> GTMGVNAVHWFRKGLRLHDNPALKECIQGADTIRCVYILDPWFAGSSNVGINRWRFLLQCLEDLDANLRKLNSRLFVIRGQPADVFPRLFKEWNITKLSIEYDSEPFGKERDAAIKKLATEAGVEVIVRISHTLYDLDKIIELNGGQPPLTYKRFQTLVSKMEPLEMPADTITSDVIGKCMTPLSDDHDEKYGVPSLEELGFDTDGLSSAVWPGGETEALTRLERHLERKAWVANFERPRMNANSLLASPTGLSPYLRFGCLSCRLFYFKLTDLYKKVKKNSSPPLSLYGQLLWREFFYTAATNNPRFDKMEGNPICVQIPWDKNPEALAKWAEGRTGFPWIDAIMTQLRQEGWIHHLARHAVACFLTRGDLWISWEEGMKVFEELLLDADWSINAGSWMWLSCSSFFQQFFHCYCPVGFGRRTDPNGDYIRRYLPVLRGFPAKYIYDPWNAPEGIQKVAKCLIGVNYPKPMVNHAEASRLNIERMKQIYQQLSRYRG

1 This clock is composed of a transcriptional regulatory network of clock genes, Period ( Per1 and Per2), Cryptochrome ( Cry1 and Cry2), Clock and Bmal1. In the core feedback loop of the mammalian circadian clock, transcription factors CLOCK and BMAL1 activate transcription of Per and Cry genes by forming a heterodimer. The translated PER and CRY proteins then repress the transcriptional activity of CLOCK-BMAL1 to close the loop, followed by the degradation of PER and CRY through the ubiquitin-proteasome pathway reactivating CLOCK-BMAL1. 31 CRY is a repressor of CLOCK-BMAL1, and CRY stabilization reduces the expression of CLOCK-BMAL1-target genes such as Per2.

In this study, we revealed the effects of a new circadian clock modulator TH401, which contains a methylbenzimidazole moiety, on CRY isoforms by taking a target-based approach. TH401 directly interacted with CRY1 and CRY2, albeit with a slight preference to CRY2, and the X-ray crystal structure of a CRY1-TH401 complex revealed the binding mode of TH401. The overall protein fold was highly similar to previously published CRY1 structures. With regard to the binding mode of TH401, the 1-methylbenzimidazole moiety formed hydrophobic interactions with W292, R293 and W399, as well as additional offset π-stacking with W292. The trimethoxyphenyl moiety formed multiple hydrophobic interactions with residues R358, A362, F381, L385, A388, W397 and L400. Oxygen atoms in two methoxy groups ( ortho and meta) formed hydrogen bonds with the guanidinium group of R358, while methyl groups in two methoxy groups ( ortho and meta) formed C–H hydrogen bonds with N393 and S396. One notable difference in the binding mode of TH401, compared to almost all other CRY-interacting compounds, was the absence of a canonical H-bond between the linker (connecting the methylbenzimidazole and trimethoxyphenyl moieties) and S396. Instead, H359 interacted with the sulfanylacetohydrazide linker by forming two hydrogen bonds, one with the hydrazide carbonyl and the other with a hydrazide nitrogen. The binding of TH401 resulted in the repositioning of the gatekeeper W399 from an intrinsic “out” conformation in CRY1-PG4 (apo-like structure) to a “middle” conformation in CRY1-TH401. The W399 “middle” conformation resulted in the loss of an NH–aryl interaction between W399 and Q407 at the gatekeeper–lid loop interface in CRY1-PG4.(1R,3S,5Z)-5-[(2E)-2-[(1R,3aS,7aR)-1-[(2R,6R)-6-(1-adamantyl)-6-oxidanyl-hex-4-yn-2-yl]-7a-methyl-2,3,3a,5,6,7-hexahydro-1H-inden-4-ylidene]ethylidene]-4-methylidene-cyclohexane-1,3-diol 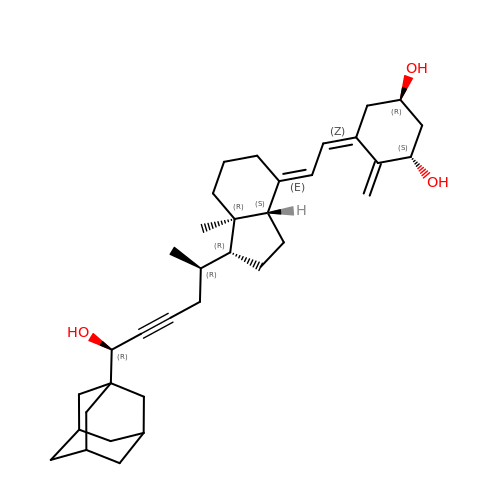| C35 H50 O3 | RKVGVUCXMUXZTG-JQIDRQNQSA-N[[(2S,3R,4S,5R)-5-(2-azanyl-6-oxidanylidene-1H-purin-9-yl)-3,4-bis(oxidanyl)oxolan-2-yl]methoxy-oxidanyl-phosphoryl] 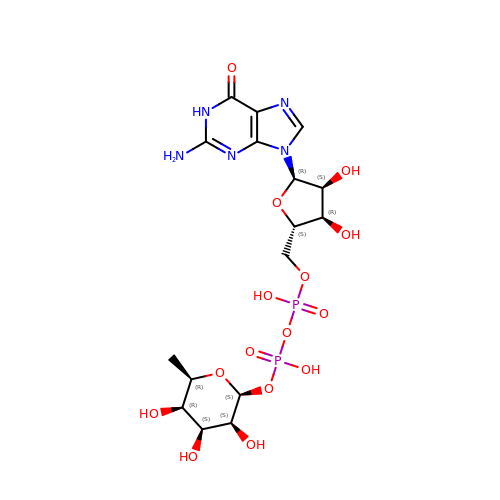[(2S,3S,4S,5R,6R)-6-methyl-3,4,5-tris(oxidanyl)oxan-2-yl] hydrogen phosphate | C16 H25 N5 O15 P2 | LQEBEXMHBLQMDB-STHOTVMKSA-N> GSPGIRMALKTDQILDKLNEKLAQVDRSKRSFTVILFVHLRQEGKVVRSVVLDFNDLKISEIELAVTS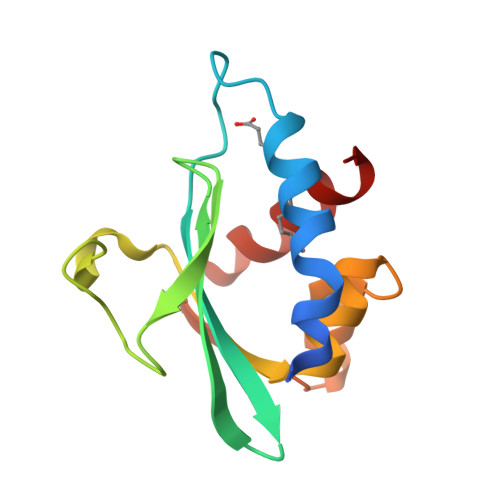TADYPAERIDASITIDDNDFYLVATKETSFAALIEQGKVDITGNKQAFLTLDEKFRNK>[2x]MSNRAKSPALDAVVIGAGVTGIYQAFLINQAGMKVLGIEAGEDVGGTWYWNRYPGCRLDTESYAY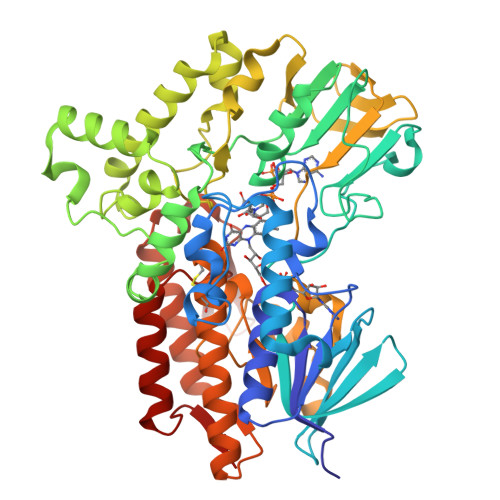GYFALKGIIPEWEWSENFASQPEMLRYVNRAADAMDVRKHYRFNTRVTAARYVENDRLWEVTLDNEEVVTCRFLISATGPLSASRMPDIKGIDSFKGESFHSSRWPTDAEGAPKGVDFTGKRVGVIGTGATGVQIIPIAAETAKELYVFQRTPNWCTPLGNSPMSKEKMDSLRNRYPTILEYVKSTDTAFPYHRDPRKGTDVSESERDAFFEELYRQPGYGIWLSGFRDLLLNKESNKFLADFVAKKIRQRVKDPVVAEKLIPKDHPFGAKRVPMETNYYETYNRDNVHLVDIREAPIQEVTPEGIKTADAAYDLDVIIYATGFDAVTGSLDRIDIRGKDNVRLIDAWAEGPSTYLGLQARGFPNFFTLVGPHNGSTFCNVGVCGGLQAEWVLRMISYMKDNGFTYSEPTQAAENRWTEEVYADFSRTLLAEANAWWVKTTTKPDGSVVRRTLVHVSGGPEYRKRCEQVAYNNYNGFELA>RRYTLNATALGLGGAATRQLTFQTSSPAHLTMPYVMPGDGEVVGVGEPVAIRFDENIADRGAAEKAIKITTNPPVEGAFYWLNNREVRWRPEHFWKPGTAVDVAVNTYGVDLGEGMFGEDNVQTHFTIGDEVIATADDNTKILTVRVNGEVVKSMPTSMGKDSTPTANGIYIVGSRYKHIIMDSSTYGVPVNSPNGYRT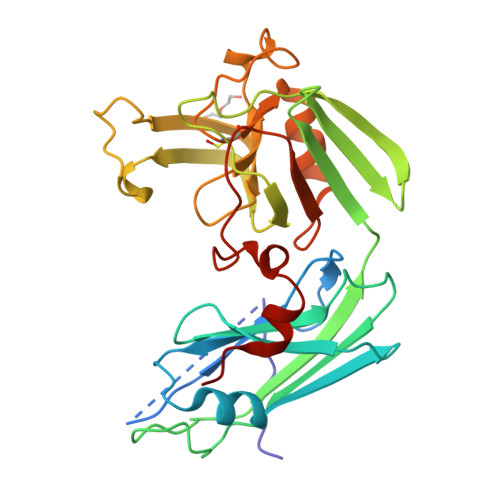DVDWATQISYSGVFVHSAPWSVGAQGHTNTSHGCLNVSPSNAQWFYDHVKRGDIVEVVNTVGGTLPGIDGLGDWNIPWDQWRAGNAKA[2x]> MENTENSVDSKSIKNLEPKIIHGSESMDSGISLDNSYKMDYPEMGLCIIINNKNFHKSTGMTSRSGTDVDAANLRETFRNLKYEVRNKNDLTREEIVELMRDVSKEDHSKRSSFVCVLLSHGEEGIIFGTNGPVDLKKIT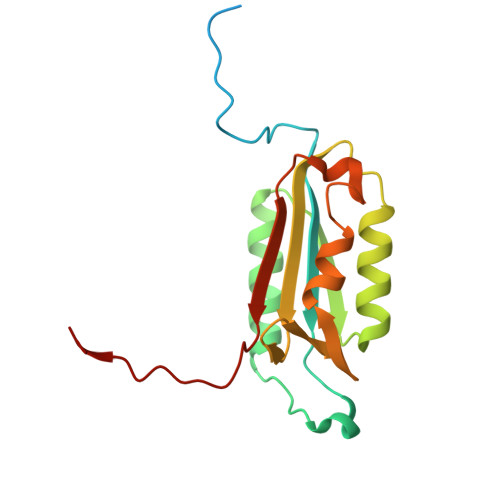NFFRGDRCRSLAGKPKLFIIQACRGTELDCGIETD>SNGLEDSSTISFITWNIDGLDGCNLPERARGVCSCLALYSPDVVFLQEVIPPYCAYLKKRAASYTIITGNEEGYFTAILLKKGRVKFKSQEIIPFPNTKMMRNLLCVNVSLGGNEFCLMTSHLESTREHSAERIRQLKTVLGKMQEAPDSTTVIFAGDTNLRDQEVIKCGGLPDNVFDAWEFLGKPKHCQYTWDTKANNNLRIPAAYKHRFDRI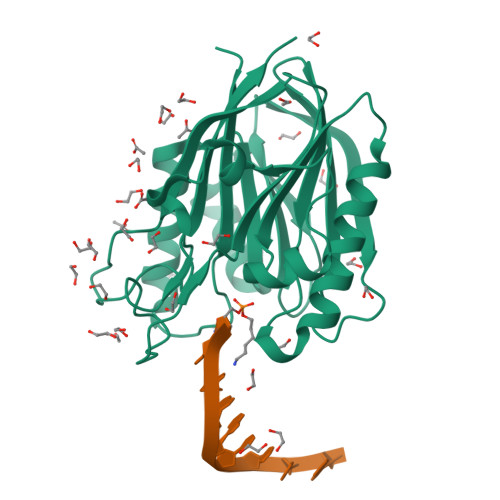FFRAEEGHLIPQSLDLVGLEKLDCGRFPSDHWGLLCTLNVVL[6x]> ASAKELACQEITVPLCKGIGYNYTYMPNQFNHDTQDEAGLEVHQFWPLVEIQCSPDLKFFLCSMYTPICLEDYKKPLPPCRSVCERAKAGCAPLMRQYGFAWPDRMRCDRLPEQGNPDTLCMDAAALEVLFQ;> AWSVNNFLMTGPKAYLTYSASVAVGAQNGIEECKYQFAWERWNCPESTLQLATHNGLRSATRETSFVHAISSAGVMYTLTRNCSMGDFDNCGCDDSRNGRIGGRGWVWGGCSDNAEFGERISKLFVDGLETGQDARALMNLHNNEAGRLAVKETMKRTCKCHGISGSCSIQTCWLQLAEFRDIGNHLKIKHDQALKLEMDKRKMRSGNSADNRGAIADAFSSVAGSELIFLEDSPDYCLKNISLGLQGTEGRE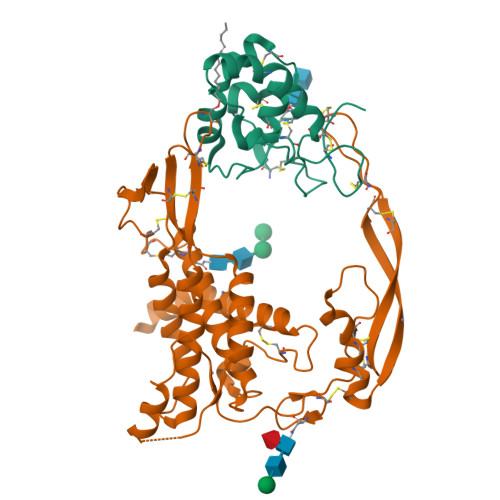CLQSGKNLSQWERRSCKRLCTDCGLRVEEKKTEIISSCNCKFHWCCTVKCEQCKQVVIKHFCA> DFR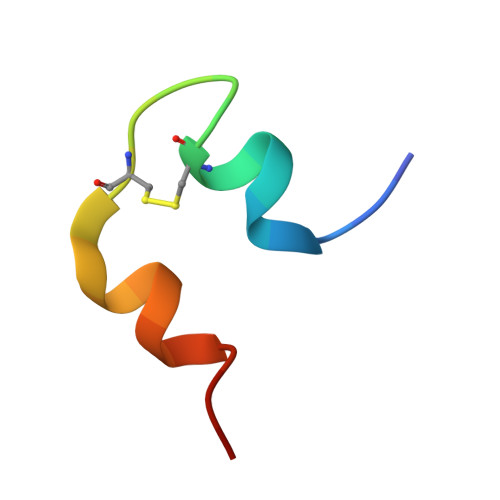GVVDSCCRNSCSFSTLRAYCDS>[2x]KPGAPWWKSAVFYQVYPRSFKDTNGDGIGDFKGLTEKLDYLKGLGIDAIWINPHYASPNTDNGYDISDYREVMKEYGTMEDFDRLMAELKKRGMRLMVDVVINHSSDQHEWFKSSRASKDNPYRDYYFWRDGKDGHEPNNYPSFFGGSAWEKDPVTGQYYLHYFGRQQPDLNWDTPKLREELYAMLRFWLDKGVSGMRFDTVATYSKTPGFPDLTPEQMKNFAEAYTQGPNLHRYLQEMHEKVFDH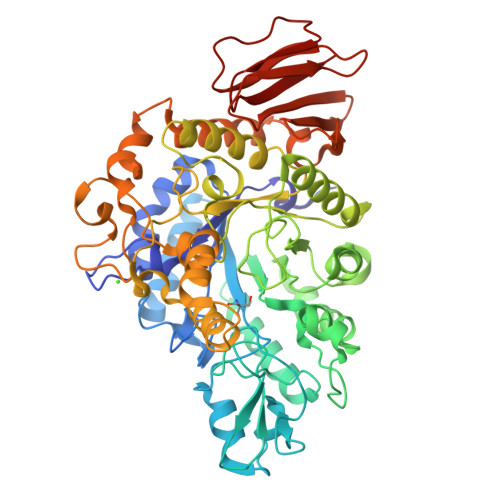YDAVTAGEIFGAPLNQVPLFIDSRRKELDMAFTFDLIRYDRALDRWHTIPRTLADFRQTIDKVDAIAGEYGWNTFFLGNHDNPRAVSHFGDDRPQWREASAKALATVTLTQRGTPFIFQGDELGMTNYPFKTLQDFDDIEVKGFFQDYVETGKATAEELLTNVALTSRNNARTPFQWDDSANAGFTTGKPWLKVNPNYTEINAAREIGDPKSVYSFYRNLISIRHETPALSTGSYRDIDPSNADVYAYTRSQDGETYLVVVNFKAEPRSFTLPDGMHIAETLIESSSPAAPAAGAASLELQPWQSGIYKVK>MLEYSELYPIQNEYRMMQSLDGMWKFQFDPEEIGKKSGWENGLPAPVSMPVPSSFADFFTDHKERDYCGDFWYETEFYLPAEWRNKKIWLRFGSITHRGTVYCNGMEITSHEGGFLPVLADISTVAKPGQVNQVVVKINNELNETSLPCGATKILNNGRKLAKPYFDFFNYSGLQRSVWVIALPEESVKDYSVDYELCGTDALVKYEVVTTGEHPVIVRLLDAEGELVAETEGKEGILQVANARLWEVRNAYLYQIVILITDGNGVLDEYREKIGIRTVRIEGTKILLNDRPVYLKGFGKHEDFPILGRGFHWGIVKRDFECLKWTNANCFRTSHYPYAEEWYQFADEEGFLIIDEVPAVGMMRSTRNFVAAGSGNYTYFFEALTVPELLKSHIADTEEMITRDKNHPSVIAWSLFNEPETITDYAYEYFKEVFAAAETYDFQSRPMTGAFEKNSKPELCKCYPLCDFICLNRYYGWYISGGPEIEEAEELFRDEMDRWKAKELNVPFVFTEFGTDTMAGLHKLPSIMWSEEYQKEYLEMNFRVFDSYEFVQGELAWNFADFQTTEGIMRVDGNHKGVFTRDRQPKAAAVVFKDR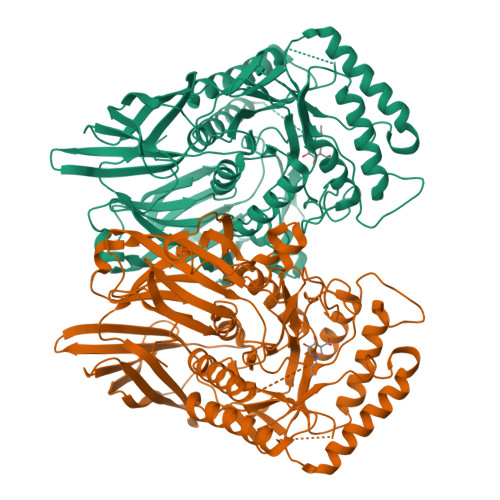WEKKNELF[2x]>[2x]MLQSLAGSSCVRLVERHR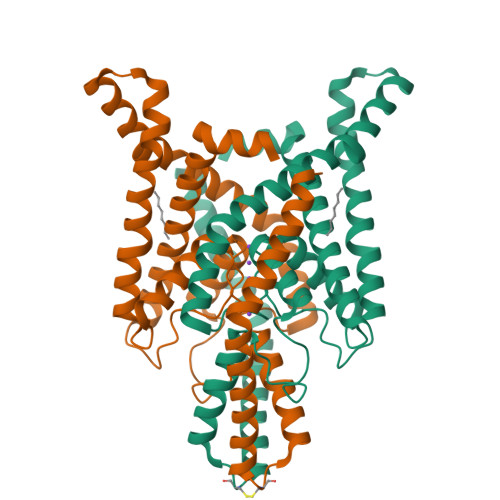SAWCFGFLVLGYLLYLVFGAVVFSSVELPYEDLLRQELRKLKRRFLEEHECLSEPQLEQFLGRVLEASNYGVSVLSNASGNWNWDFTSALFFASTVLSTTGYGHTVPLSDGGKAFCIIYSVIGIPFTLLFLTAVVQRVTVHVTRRPVLYFHIRWGFSKQVVAIVHAVLLGFVTVSCFFFIPAAVFSVLEDDWNFLESFYFCFISLSTIGLGDYVPGEGYNQKFRELYKIGITCYLLLGLIAMLVVLETFCELHELKKFRKMFYVKKDKDEDQVHIMEHDQLSFSSITEQAAGLKEEQKQNEPFVASQSPPYEDGSANH> GAMVPKASGTSGPAKQEKQSIITPADLLENMSPGWNLGN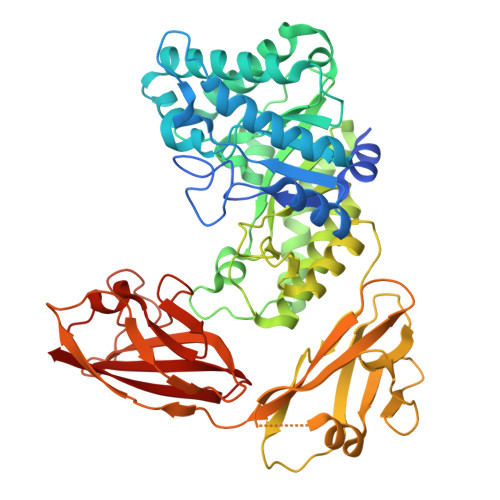TLDAVPTEGSWNNPPVREHTFDDIRDAGFKSVRIPVTWDSHIGSAPEYPIDTDWMNRVEEVTDWALEREFYVVLNIHHDSWLWISRMGNSQQETLDKLGKVWKQIAERFKNKSERLLFEIVNEPTGMSAYQMNLLNREMLNIIRSTGGKNGQRLVIVGGLEDNKDELLHSFEPPDDDRIVLTYHYYSPWDYVSNWWGRTTWGSAAEISEMEEDIKPVYEKFVREGYPVIIGEYGTLGANEKHSKWLYHDTFVRLAHKYQMVPMWWDNGNDQFDRAERQWRDPVVKEIVIQAGRGVPNAIIKPADLFIKKGQSISDQTVDIQLNGNVLTGIYQKSEPLKEGSDYTVDNAGKTVSIKASCLAKLLNGAGQPGVKAQLTFTFHKGASQVMDIILYDDPKLEKSEFTISQSAISGDLKIPASLNGTKLATVKGVVDSTGRPVLEEVWSWTPYLNYDEDFYEKDGDLYLKERVLKYLKSDSTFTFELWPKGVEAVVKVKITP>[2x]VSVITSEMKIEVRMEGAVNGHKFVITGKGSGQPFEGIQNVDLTVIEGGPLPFAFDILTTAFHYGNRVFVKYPEEIVDYFKQSFPEGYSWERSMSYEDGGICLATNNITMKKDGSNCFVNE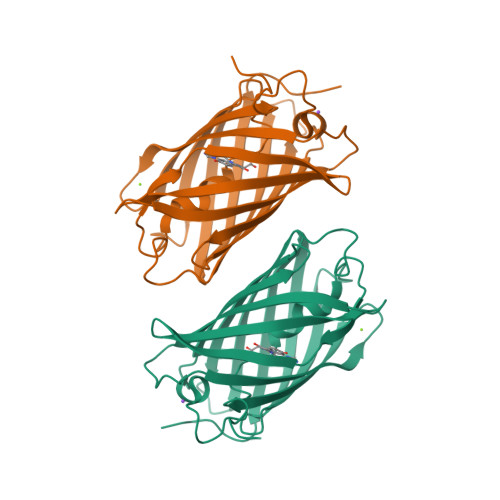IRFDGVNFPANGPVMQRKTVKWESSTEKMYVRDGVLKGDVNMALLLQGGGHYRCDFRTTYKAKKVVQLPDYHFVDHLMEITSHDKDYNKVKLYEHAKAHSGLPRLAK> IAPLVGVGLAAGAVGVGWALREFEIVGSDAPPEGLTADALKQQVYQTAKTRKSTNASTIVDNQNILDGVKHTAYTDAKIAAIEELNAGSAESAVLDAATTEVNSYLTTVQSNFLKTWNESVAELDSILSTVVNHPDIGKGDVFLMLNGSDNTIEDLLANPSGSTDATSFTLADGTTMSVGTVEVDRGTESYYYDPMSGLVGDLGDLKNGGPTVQYDGDSLVYLNASNWKPIYDEMDTVLQNVRSGISTWVSNVYGDVQSGEIEVSDLVTPRERAAMMAQEEGMSQAIADLIALNVPVDAEREATITIQDTGATLPGTFALTDASDGPLESGKTYDPSTFSGDVYFTADMSLVEGDWTAYQSGVDGGNVTLTSEPYSGTAVELNTAANETVAVDAGNWTATGNGTWYHDVSPELETDITSIESARFLSTAEQTQYETIQLQGSFTIDKLTNTQTGEEVTATSFDSS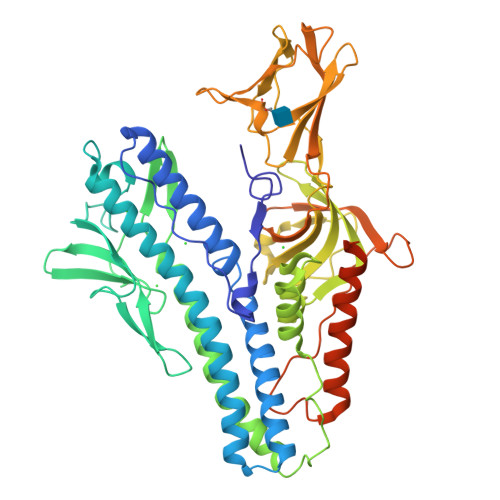EPHTDSNYITQEEWDQLEQQNKELIEKYEQSQSGGGLDLGQFDMFGIPGEIVAVGVAALVGLGVLGNN>[2x]MAKAHIELTINGHPVEALVEPRTLLIHFIREQQNLTGAHIGCDTSHCGACTVDLDGMSVKSCTMFAVQANGASITTIEGMAAPDGTLSALQEGFRMMHGLQCGYCTPGMIMRSHR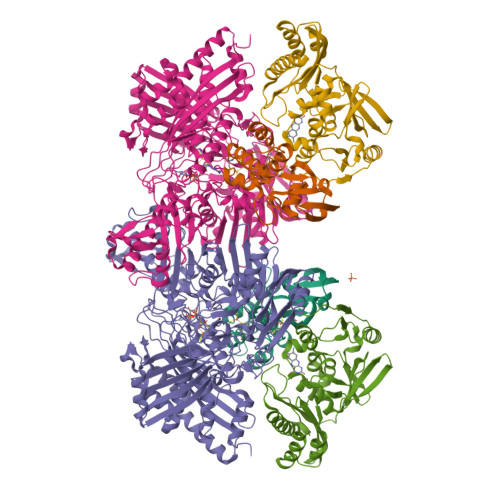LLQENPSPTEAEIRFGIGGNLCRCTGYQNIVKAIQYAAAKINGVPFEEAAE;>[2x]MNIQTTVEPTSAERAEKLQGMGCKRKRVEDIRFTQGKGNYVDDVKLPGMLFGDFVRSSHAHARIKSIDTSKAKALPGVFAVLTAADLKPLNLHYMPTLAGDVQAVLADEKVLFQNQEVAFVVAKDRYVAADAIELVEVDYEPLPVLVDPFKAMEPDAPLLREDIKDKMTGAHGARKHHNHIFRWEIGDKEGTDATFAKAEVVSKDMFTYHRVHPSPLETCQCVASMDKIKGELTLWGTFQAPHVIRTVVSLISGLPEHKIHVIAPDIGGGFGNKVGAYSGYVCAVVASIVLGVPVKWVEDRMENLSTTSFARDYHMTTELAATKDGKILAMRCHVLADHGAFDACADPSKWPAGFMNICTGSYDMPVAHLAVDGVYTNKASGGVAYRCSFRVTEAVYAIERAIETLAQRLEMDSADLRIKNFIQPEQFPYMAPLGWEYDSGNYPLAMKKAMDTVGYHQLRAEQKAKQEAFKRGETREIMGIGISFFTEIVGAGPSKNCDILGVSMFDSAEIRIHPTGSVIARMGTKSQGQGHETTYAQIIATELGIPADDIMIEEGNTDTAPYGLGTYGSRSTPTAGAATAVAARKIKAKAQMIAAHMLEVHEGDLEWDVDRFRVKGLPEKFKTMKELAWASYNSPPPNLEPGLEAVNYYDPPNMTYPFGAYFCIMDIDVDTGVAKTRRFYALDDCGTRINPMIIEGQVHGGLTEAFAVAMGQEIRYDEQGNVLGASFMDFFLPTAVETPKWETDYTVTPSPHHPIGAKGVGESPHVGGVPCFSNAVNDAYAFLNAGHIQMPHDAWRLWKVGEQLGLHV;>[2x]MIPGSFDYHRPKSIADAVALLTKLGEDARPLAGGHSLIPIMKTRLATPEHLVDLRDIGDLVGIREEGTDVVIGAMTTQHALIGSDFLAAKLPIIRETSLLIADPQIRYMGTIGGNAANGDPGNDMPALMQCLGAAYELTGPEGARIVAARDYYQGAYFTAIEPGELLTAIRIPVPPTGHGYAYEKLKRKIGDYATAAAAVVLTMSGGKCVTASIGLTNVANTPLWAEEAGKVLVGTALDKPALDKAVALAEAITAPASDGRGPAEYRTKMAGVMLRRAVERAKARAKN In plant biosynthesis, the formation of glycosidic bond is usually catalyzed by uridine diphosphate-dependent glycosyltransferases (UGTs). In this work, we report an efficient phenolic apiosyltransferase GuApiGT from G. uralensis, and dissect mechanisms for its sugar donor selectivity towards UDP-Api through crystal structure analysis, theoretical calculations, and mutagenesis. GuApiGT could efficiently and regio-selectively catalyze 2″-O-apiosylation of flavonoid glycosides, and showed strict sugar donor selectivity towards UDP-Api. This selectivity was highly related with the unique 45-amino acid PSPG box and the key RLGSDH sugar binding motif. Through theoretical calculations and rational design, we altered the sugar donor selectivity of GuApiGT and Sb3GT1.

To further prove the critical role of the RLGSDH motif in UDP-Api selectivity, we conducted site-directed mutagenesis of Sb3GT1. Based on structural analysis, we inserted a serine residue into the motif and constructed the 375S/Q377H mutant of Sb3GT1, as well as the F372R/Q376H and F372R/375S/Q377H mutants. All the three mutants could catalyze kaempferol into its 3-O-apioside, according to the characteristic [Y0-H]- ion at m/z 284 in LC/MS analysis. We further solved the crystal structure of Sb3GT1 375S/Q377H mutant in complex with UDP-Glc at 1.43 Å resolution. The motif structure of the mutant was larger than that of WT, which may be critical for the sugar donor selectivity towards UDP-Api.

> MVFQSHIGVLAFPFGTHAAPLLTVVQRLATSSPHTLFSFFNSAVSNSTLFNNGVLDSYDNIRVYHVWDGTPQGQAFTGSHFEAVGLFLKASPGNFDKVIDEAEVETGLKISCLITDAFLWFGYDLAEKRGVPWLAFWTSAQCALSAHMYTHEILKAVGSNGVGETAEEELIQSLIPGLEMAHLSDLPPEIFFDKNPNPLAITINKMVLKLPKSTAVILNSFEEIDPIITTDLKSKFHHFLNIGPSILSSPTPPPPDDKTGCLAWLDSQTRPKSVVYISFGTVITPPENELAALSEALETCNYPFLWSLNDRAKKSLPTGFLDRTKELGMIVPWAPQPRVLAHRSVGVFVTHCGWNSILESICSGVPLICRPFFGSDHKLNSRMVEDSWKIGVRLEGGVLSKTATVEALGRVMMSEEGEIIRENVNEMNEKAKIAVEPKGSSFKNFNKLLEIINAPQSS~{N}-[7-imidazol-1-yl-2,3-bis(oxidanylidene)-6-(trifluoromethyl)-4~{H}-quinoxalin-1-yl]benzamide 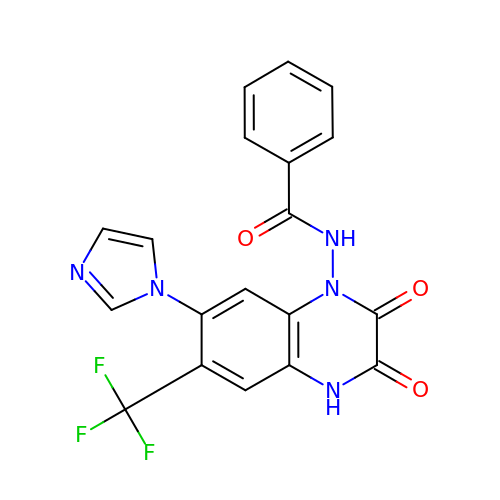| C19 H12 F3 N5 O3 | IOLCYQPDALFXJR-UHFFFAOYSA-N> DKKVDLVYMNWDSEVASINVLTQAMKEHGFDVKTTALDNAVAWQTVANGQADGMVSAWLPNTHKTQWQKYGKSVDLLGPNLKGAKVGFVVPSYMNVNSIEDLTNQANKTITGIEPGAGVMAASEKTLNSYDNLKD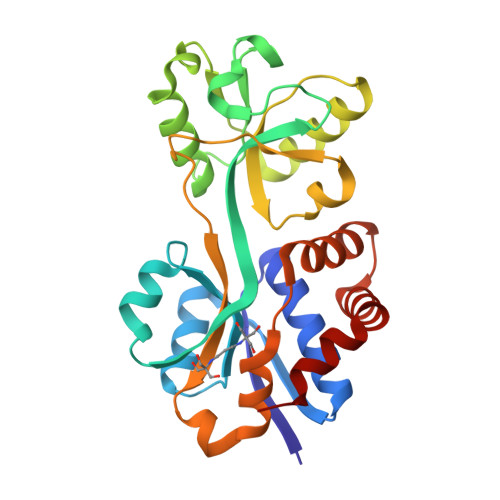WKLVPSSSGAMTVALGEAIKQHKDIVITGWSPHWMFNKYDLKYLADPKGTMGTSENINTIVRKGLKKENPEAYKVLDKFNWTTKDMEAVMLDIQNGKTPEEAAKNWIKDHQKEVDKWFKGS>[10x]GGCGAGGAA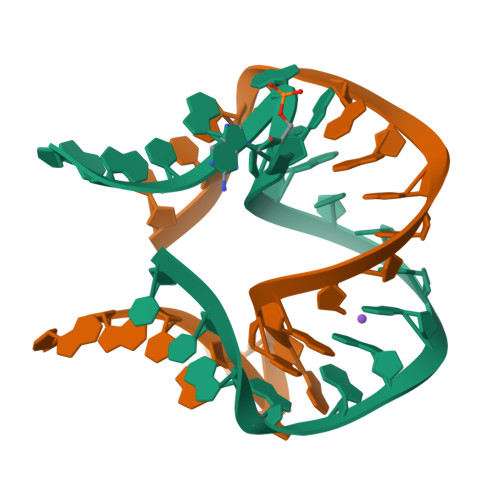CCGGGGAGCC> GSFDLDDVQPNKAVEPEKTKVNYTDEETQKRKKEELDKLMEPALGYVTKIPVNIPSVRKTEISEIDTVTDESLSLVPNEDKLRTIANENYGSVVTKSGSNTMNFVRSGYTIDV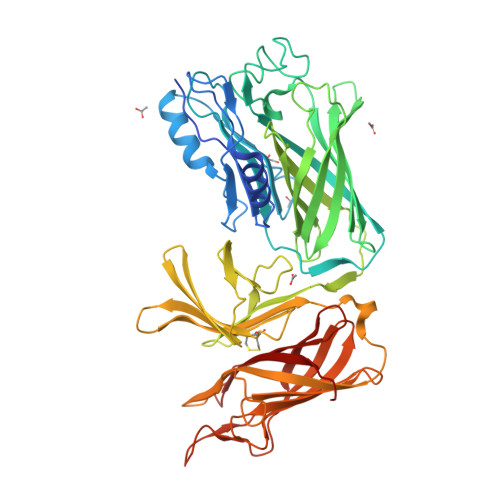VHYGLRDKGYVYYKGVHPSKELPKGNIIVYQGEWDFTSNADLDAKRPNYNPEFNGAGAGQRVGVTSADAKERTYISKFNIDFSNKKLNGQLLTKTKENQEKLRYTVEANISGNRFRGKATATDKTDPILGKDSEHLEGGLYGPKSEELAGKFVAHDKSLFAVFSGKRGNDVLETVKIIDASKIDLTTFESSELNNFGNANVLIIDGQKIDLAGADFKNRKTVDINGKTMVAIACCSNLEYMKFGQLWQKEGEQTKDNSLFLQGERTATDKIPVGGNYKYVGTWDALVSKGTNWVAEADNNRESGYRSEFDVNFGDKKVSGKLFDKGGIVPVFMINADIKGNGFTGTANTTDTGFALDSGSSQHGNAVFSDIKVNGGFYGPTAGELGGQFHHKSDNGSVGAVFGAKRQIEK>[2x]GSHGMRVIIAGFGRFGQITGRLLLSSGVKMVVLDHDPDHIETLRKFGMKVFYGDATRMDLLESAGAAKAEVLINAIDDPQTNLQLTEMVKEHFPHLQIIARARDVDHYIRLRQAGVEKPERET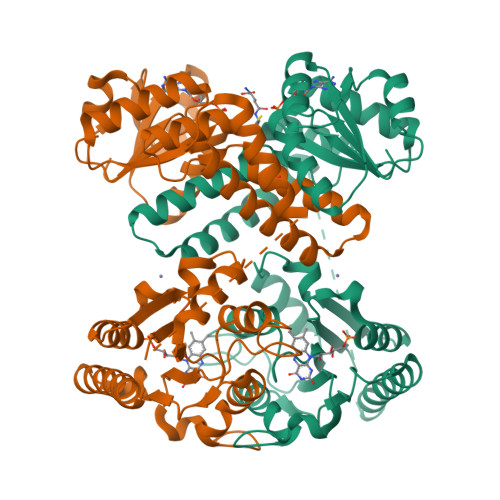FEGALKTGRLALESLGLGPYEARERADVFRRFNIQMVEEMAMVENDTKARAAVYKRTSAMLSEIITEDREHLSLIQRHGWQGTEEGKHTGNMADEPETKPSSTSGGLVPRGSSGMILIIYAHPYPHHSHANKRMLEQARTLEGVEIRSLYQLYPDFNIDIAAEQEALSRADLIVWQHPMQWYSIPPLLKLWIDKVFSHGWAYGHGGTALHGKHLLWAVTTGGGESHFEIGAHPGFDVLSQPLQATAIYCGLNWLPPFAMHCTFICDDETLEGQARHYKQRLLEWQEAHHG Human RAD52 (RAD52) is a DNA-binding protein involved in many DNA repair mechanisms and genomic stability maintenance. Full-length RAD52 (FL-RAD52) is a protein of 418 amino acids, but it is not stable in its monomeric form. FL-RAD52 physiological form is promoted by the association of the N-terminal portions (212 amino acids each) of multiple FL-RAD52 molecules arranged in a ring-shaped structure on which DNA wraps around. The C-terminal domains of the associated monomeric units, whose structural organization has been elusive to date, contain two binding sites for DNA repair protein RAD51 homolog 1 (RAD51) and replication protein A (RPA).

Here, we report the 2.2 Å resolution cryo-EM reconstruction of the full-length RAD52 (FL-RAD52) protein. Despite our extensive data analysis, no minor 2D or 3D classes corresponding to alternative ring organizations were detected. The c11 symmetry was therefore applied, allowing to obtain an electron density map of the FL-RAD52 at 2.2 Å average resolution (0.143 FSC correlation criterion) higher than without imposing any symmetry (2.4 Å and 2.7 Å). As observed in other structures of RAD52 N-terminal, our model comprises a mushroom-like closed ring composed of a stem region formed by the β-β-β-α fold of each monomer (residues 79–156), and by a domed cap region at both the N- and C-terminal of the stem region, that ends with a flat top. Most amino acid side chains between serine (Ser) 25 and cysteine (Cys) 208 were well resolved and clearly recognizable. Interestingly, densities at the N- (residues 1–22) and C-terminus (residues 209–430) were largely absent. Densities corresponding to 498 water molecules, equivalent to about 45 water molecules per protomer, were identified in our cryo-EM map. These water molecules are connected to the protein ring by hydrogen bonds and coordinate to FL-RAD52 single or multiple polar residues and to the polypeptide backbone, also forming connected chains. In summary, this analysis allowed the identification of a water molecules network that stabilizes not only each protomer unit, but also the protomer-protomer interactions, i.e., the overall N-terminal ring structure. In addition, in our 3D structure, several water molecules were also observed at the inner DNA binding site of FL-RAD52. In this region, several key residues, known to electrostatically interact with the phosphate backbone of the ssDNA, namely lysine (Lys) 152, arginine (Arg) 153 and (Arg) 156 are involved in water-mediated hydrogen bonds. The position of Arg55 in our model is clearly not compatible with the binding of the ssDNA to the inner DNA binding site, suggesting that this residue may also work as an entry/exit gate for ssDNA in the first phases of FL-RAD52-ssDNA interaction, not only during homology search.

>[11x]MHHHHHHENLYFQGMSGTEEAILGGRDSHPAAGGGSVLCFGQCQYTAEEYQAIQKALRQRLGPEYISSRMAGGGQKVCYIEGHRVINLANEMFGYNGWAHSITQQNVDFVDLNNGKFYVGVCAFVRVQLKDGSYHEDVGYGVSEGLKSKALSLEKARKEAVTDGLKRALRSFGNALGNCILDKDYLRSLNKLPRQLPLEVDLTKAKRQDLEPSVEEARYNSCRPNMALGHPQLQQVTSPSRPSHAVIPADQDCSSRSLSSSAVESEATHQRKLRQKQLQQQFRERMEKQQVRVSTPSAEKSEAAPPAPPVTHSTPVTVSEPLLEKDFLAGVTQELIKTLEDNSEKWAVTPDAGDGVVKPSSRADPAQTSDTLALNNQMVTQNRTPHSVCHQKPQAKSGSWDLQTYSADQRTTGNWESHRKSQDMKKRKYDPS N-hydroxy-4-[(1H-indol-1-yl)methyl]benzamide | C16 H14 N2 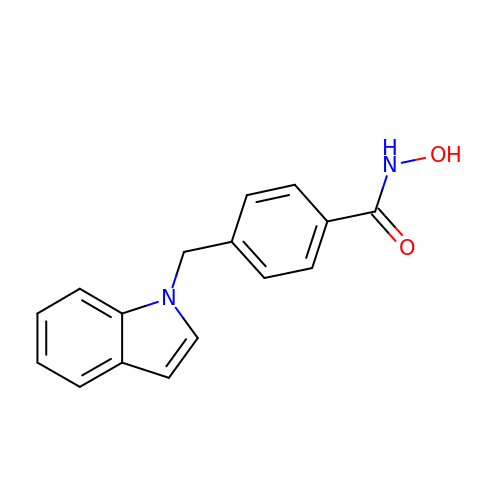O2 | SUWMPMSWSJBENV-UHFFFAOYSA-N> MNHKVHHHHHHHHMSQWYELQQLDSKFLEQVHQLYDDSFPMEIRQYLAQWLEKQDWEHAANDVSFATIRFHDLLSQLDDQYSRFSLENNFLLQHNIRKSKRNLQDN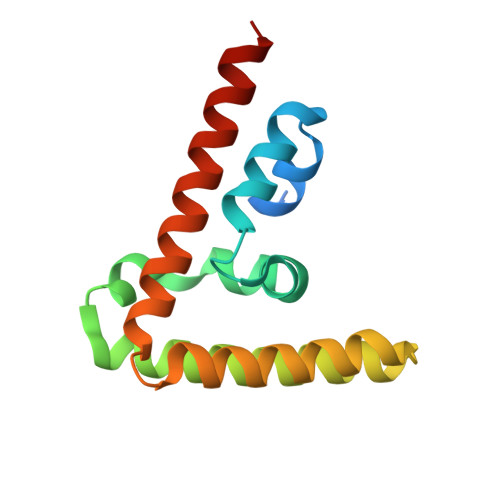FQEDPIQMSMIIYSCLKEERKILENAQRFNQAQ>MLKPNVAIIVAALKPALGIGYKGKMPWRLRKEIRYFKDVTTRTTKPNTRNAVIMGRKTWESIPQKFRPLPDRLNIILSRSYENEIIDDNIIHASSIESSLNLVSDVERVFIIGGAEIYNELINNSLVSHLLITEIEHPSPESIEMDTFLKFPLESWTKQPKSELQKFVGDTVLEDDIKEGDFTYNYT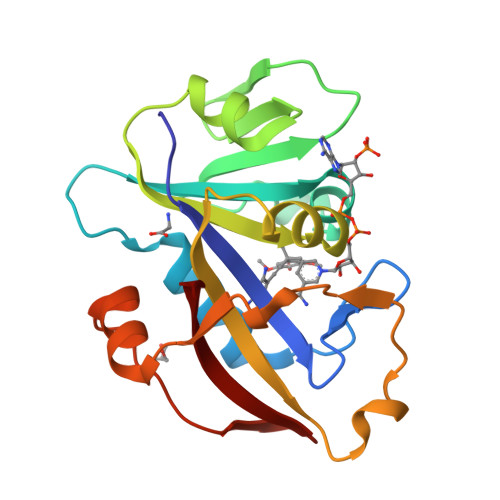LWTRK[2x]>DLMFTEMRAESWLRGSGSSGASLLQILNVRVVGSGERVVVLSHGFGTDQSAWSRVLPYLTRDHRVVLYDLVCAGSVNPDHFDFRRYDNLDAYVDDLLAILDALRIPRCAFVGHSVSAMIGILASIRRPDLFAKLVLIGASPRFLNDSDYHGGFELEEIQQVFDAMGA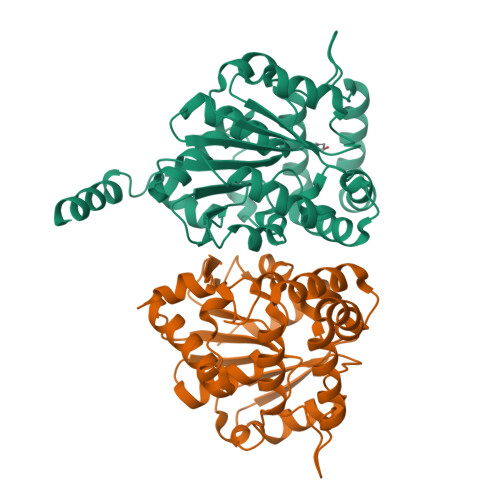NYSAWATGYAPLAVGADVPAAVQEFSRTLFNMRPDISLHVCQTVFKTDLRGVLGMVRAPCVVVQTTRDVSVPASVAAYLKAHLGGRTTVEFLQTEGHLPHLSAPSLLAQVLRRALARY[8x]1-[3-(1H-pyrrol-1-yl)phenyl]methanamine | 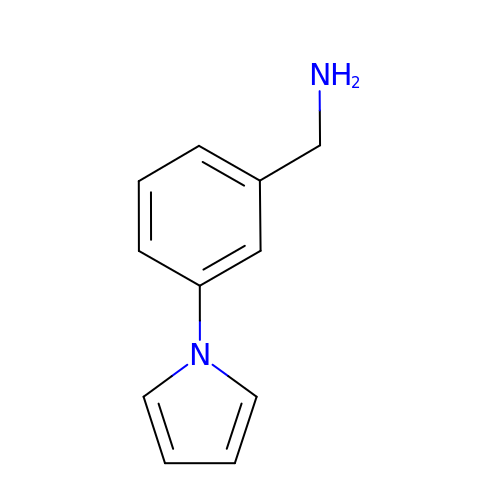C11 H12 N2 | XLBYUDUEHVKUKQ-UHFFFAOYSA-N>MHHHHHHHMSKAFIGKPAPDFATKAVFDGDFVDVKLSDYKGKYVVLFFYPLDFTFVCPTEIIAFSDRFPEFKNLNVAVLACSTDSVFSHLAWINTPRKHGGLGDMKIPVLADTNHQIAKDYGVLKDDEGIAYRGLFI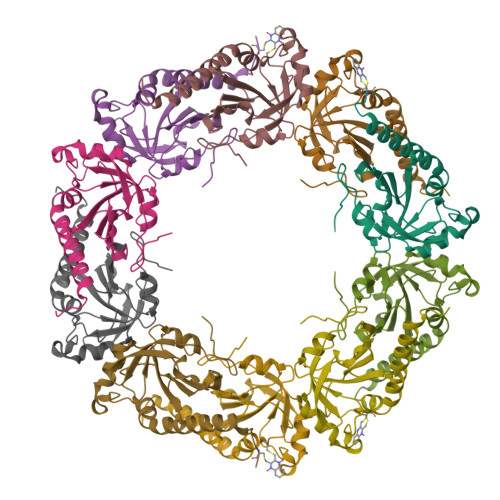IDPKGILRQITINDLPVGRSVDETLRLVQAFQYTDKHGEVCP[5x]>[2x]DVVDPDIFNRDPRDHYDLLQRLGGGTYGEVFKARDKVSGDLVALKMVKMEPDDDVSTLQKEILILKTCRHANIVAYHGSYLWLQKLWICMEFCGAGSLQDIYQVTGSLSELQISYVCREVLQGLAYLHSQKKI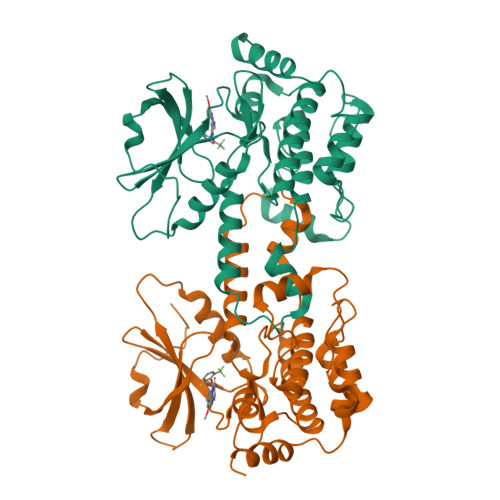HRDIKGANILINDAGEVRLADFGISAQIGAELARRLEFIGTPYWMAPEVAAVALKGGYNELCDIWSLGITAIELAELQPPLFDVHPLRVLFLMTKSGYQPPRLKEKGKWSAAFHNFIKVTLTKSPKKRPSATKMLSHQLVSQPGLNRGLILDLLDKLKNP> TCNIKNGRCEQFCKNSADNKVVCSCTEGYRLAENQKSCEPAVPFPCGRVSVSQTSKLTR;> F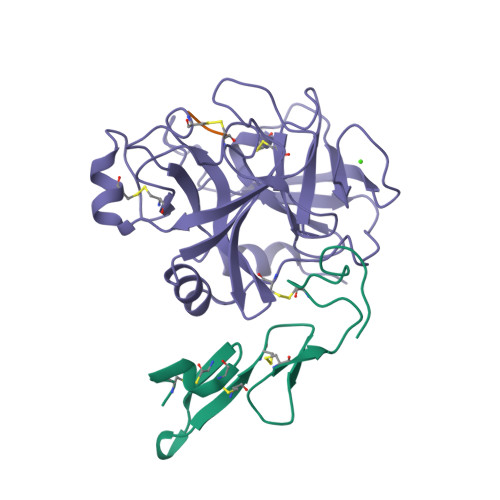PR;> VVGGEDAKPGQFPWQVVLNGKVDAFCGGSIVNEKWIVTAAHCVETGVKITVVAGEHNIEETEHTEQKRNVIRIIPHHNYNAAINTYNHDIALLELDEPLVLNSYVTPICIADKEYTNIFLKFGSGYVSGWGRVFHKGRSALVLQYLRVPLVDRATCLRSTKFTITNNMFCAGFHEGGRDSCQGDSGGPHVTEVEGTSFLTGIISWGEECAMKGKYGIYTKVSRYVNWIKEKTKLT>GMRKDDVVIVTCAITGAIHTPSMSPYLPVTPDQIVEEAVKAAEAGAGMVHIHARDPKDGRPTTDVEVFRYICREIKKQSDVVINVTTGGGGTLGIPVEERAKVVPALKPEIATFNMGSMNFAIHPLLKKYKEFKYDWEPEYLEMTRDIVFRNTFKDLEALSRIFKENDTKPELECYDIGQIYNTAFMFHEGYLEPPLRLQFIHGILGGIGTAVEDVLFMKQTADRLIGRENYTWSLVGAGRFQMPLGTLAVIMGGDVRVGLEDSLYIERGKLAKSNAEQVEKMVRI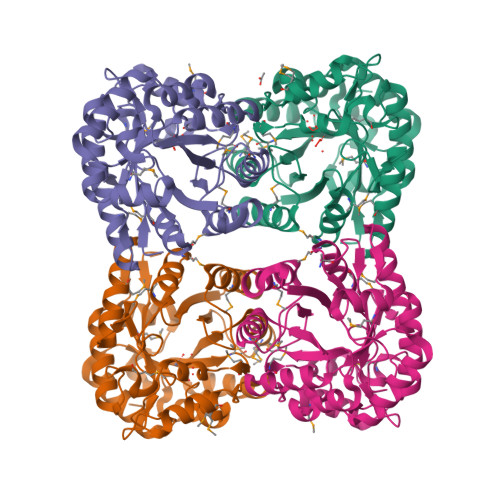VKELGKRPATPDEVREILGLKGKERVNF[4x]> MNIVITGAKGFVGKNLKADLTSTTDHHIFEVHRQTKEEELESALLKADFIVHLAGVNRPEHDKEFSLGNVSYLDHVLDILTRNTKKPAILLSSSIQATQDNPYGESKLQGEQLLREYAEEYGNTVYIYRWPNLFGKWCKPNYNSVIATFCYKIARNEEIQVNDRNVELTLNYV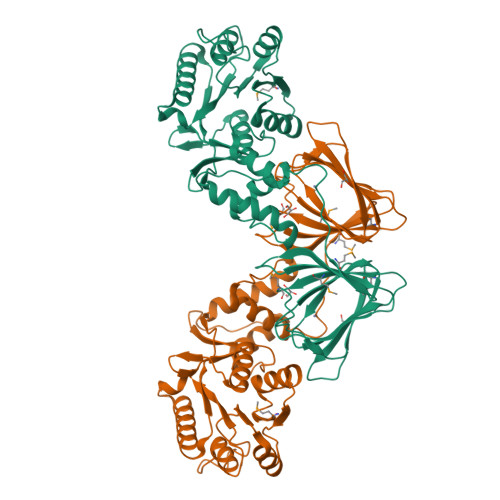DDIVAEIKRAIEGTPTIENGVPTVPNVFKVTLGEIVDLLYKFKQSRLDRTLPKLDNLFEKDLYSTYLSYLPSTDFSYPLLMNVDDRGSFTEFIKTPDRGQVSVNISKPGITKGNHWHHTKNEKFLVVSGKGVIRFRHVNDDEIIEYYVSGDKLEVVDIPVGYTHNIENLGDTDMVTIMWVNEMFDPNQPDTYFLEV>[2x]TTNKPIVLSTWNFGLHANVEAWKVLSKGGKALDAVEKGVRLVEDDPTERSVGYGGRPDRDGRVTLDACIMDENYNIGSVACMEHIKNPISVARAVMEKTPHVMLVGDGALEF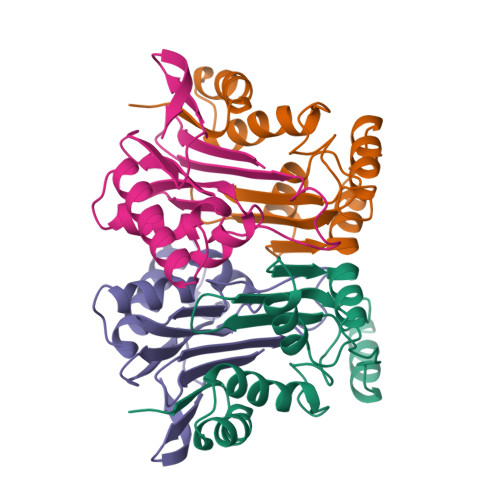ALSQGFKKENLLTAESEKEWKEWLKTSQYKPIVNIENHD;>CIGMIALDAQGNLSGACTTSGMAYKMHGRVGDSPIIGAGLFVDNEIGAATATGHGEEVIRTVGTHLVVELMNQGRTPQQACKEAVERIVKIVNRRGKNLKDIQVGFIALNKKGEYGAYCIQDGFNFAVHDQKGNRLETPGFALK[2x]>[2x]Q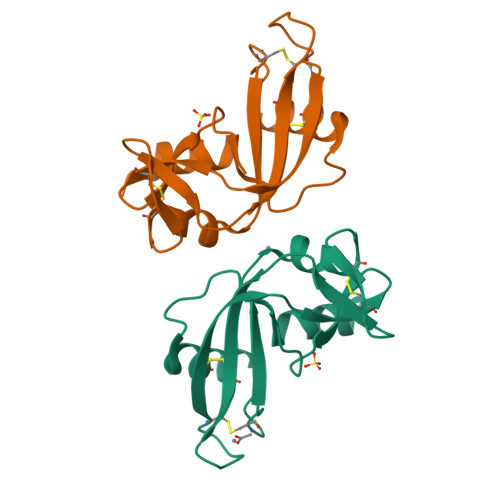DNYRYIKFLTQHYDAKPTGRDYRYCESMMKKRKLTSPCKEVNTFIHDTKNNIKAICGENGNPYGVNFRISNSRFQVTTCTHKGGSPRPPCQYNAFKDFRYIVIACEDGWPVHFDESFISP>MGNDWNPESFAIDEFMNTTDDIWVLNTTQQNPQACKKDKKHNITENGIYFFRSHKENGQIKTQTLFGEFIHFSEEEKVNNRISISDESSGVHAEHLYYSSEDKKCGLVQVFAKDQNVWTELRVRGHPNYGSLDAGCRREYEAYVKEIKGKKNSTSPYSDDCQIKV[8x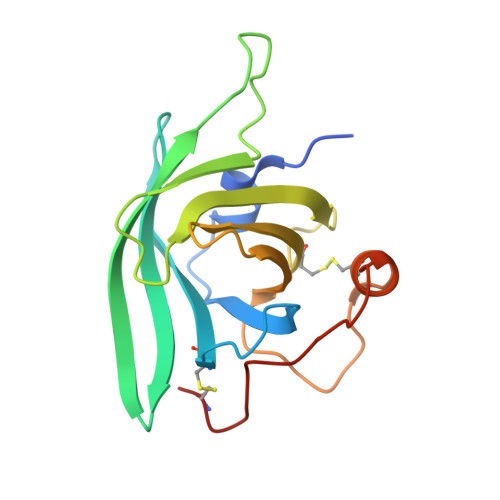]> KAVTDMDINELRKLMIGKAII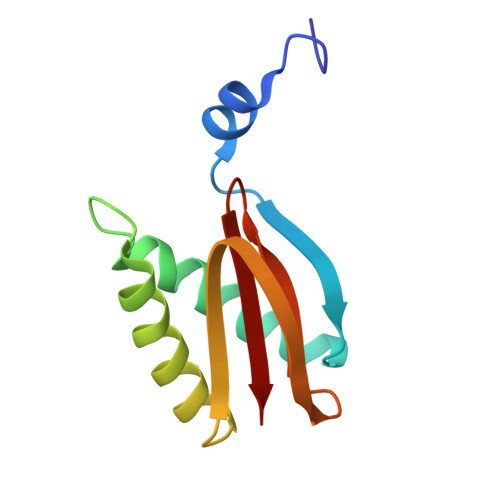NSSDMQGDLLQEAQDVIQSGIENNSAPVLNIEAACKYIKENLDKKFGPTWQCIIGEGYAYDVTVQNNTLLFMFYNGNLAVLIFKS>MAYAQWVIIIIHNVGSQDVKIKNLKASWGKLHADGDKDAEVSASNYEGKIVKPDEKLQIN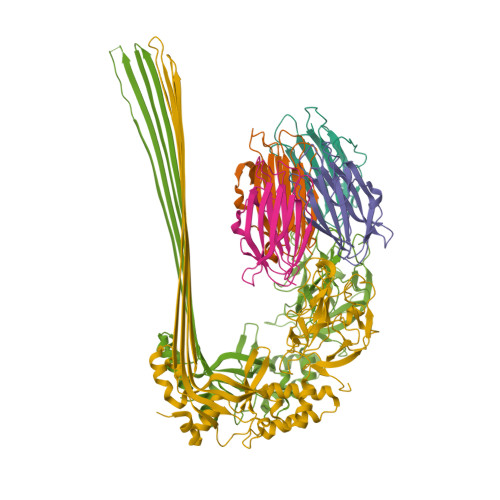ASGRSDAAEGTTGTFDLVDPADGDKQVRHFYWDSPWGSKTNTWTVSGSNTKWMIEYSGQNLDSGALGTITVDTLKKGENLYFQ[4x];>HHHHHHHHSQAGDTLNDVIQDPTRRNKLINDNNLLKGIIMGRDGPVPSSRELIVRPDTLRAIINNRATIETTTMEAEFTETLMESNYNSASVKVSAPFITANSEYSESSSFKNTETEKSMYTSSRYLFPQGRIDFTTPDSGFDDVIKLSPQFTSGVQAALAKATGTEKREALQNLFQEYGHVFRTKVHIGGVLSAHTMETFSRSENETEVKQDVKAGLEGAVKGWGGGATAGHGNTQGTITTSQNRKLNVKYIVNGGDYTKIQNTEEWVASTNQSEHWRVIEVTEVTAVADLLPQPIRGQVKDLLKPLLGKWVDVEKVPGLESLPVSVYRPKGAIPAGWFWLGDTADASKALLVKPTLPARSGRNPALTSLHQGSGMTEQPFVDLPQYQYLSTYFGSFAHDTPPGSTLRGLRPDHVLPGRYEMHGDTISTAVYVTRPVDVPFPEDECFDLKSLVRVKLPGSGNPPKPRSALKKSMVLFDSGEK[2x]> MGSPTNRLNAVQRQHLDQALAWLRGCVAPTADLRLDSREIEPGDVFVACPGLASDGRQFMDQALARGASAILYETEGASVAPVGAQALPVAQLRTLLGALADEWYGRPSQDLSVVAITGTNGKTSCTQWLAQVLTRMGKPCGSIGTLGALLPDGQSLGGSLTTPDVLTMHRTLARMRAAGARAVALEASSIGIEQGRLDHIRIAVAGFTNLTRDHLDYHGTMQRYEQAKAALFQWPDLQAAVVNADDPAGERLLASLPAALKTGYSLQGAPADVHARDLQATAHGQVFTLALPDGEAQIVTRLLGQHNISNLLLVAGALSKLGWPLPQIARELAAISPVDGRLQAVTPVPLQHLTAGAQGALVVVDYAHTPDALARALTALRPVAQARGGRLVCVFGCGGER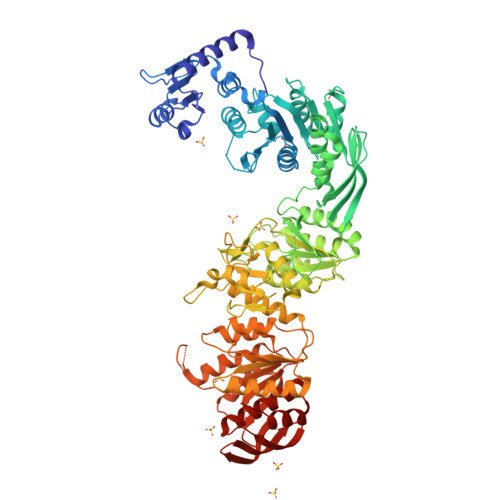DPGKRPEMGRIAVERADRVVVTSDNPRSESPQDIIDQILAGIPAGMRAAVQPDRALAIMQTLWSAAPDDVILLAGKGHETYQDIGGRKLPFDDRQWARLALLLPHAGAVSTDTRRIGRGELFVALSGENFDGHDYLPQAQSAGACAAVVAHPVADVALPQLVLGDTLAALGRMGTAWRSSFTLPVVAVTGSNGKTTTKEMISAILAQWQGDDGRLATAGNFNNEIGVPLTLLRLRARHRAAVFELGMNHPGEIERLAAMAAPTVALVTNAQREHQEFMHTVEAVAHENGAVIGALPEDGVAVYPGDEPYAAIWDKLAGARRVLRFGLQPGLDVYAERVVTQAHGTQCGVVTPAGSAGLDLPVPGLHNLRNALAAIACGLAAGAPLHTCIAALAGFQAVAGR> QNVGKWGPMVKFPVVPVAVALVPETGNLLVWSSGWPNRWTTAGNGKTYTSLYNVNTGNISDAIVQNTQHDMFCPGTSLDADGRIIVTGGSSAAKTSVLDFKKGESSPWTPLSNMQISRGYQSSCTTSEGKIFVIGGSFSGAGTRNGEVYDPKANTWTKLAGCPVKPLVMQRGMFPDSHAWLWSWKNGSVLQAGPSKKMNWYDTKGTGSNTPAGLRGTDEDSMCGVSVMYDAVAGKIFTYGGGKGYT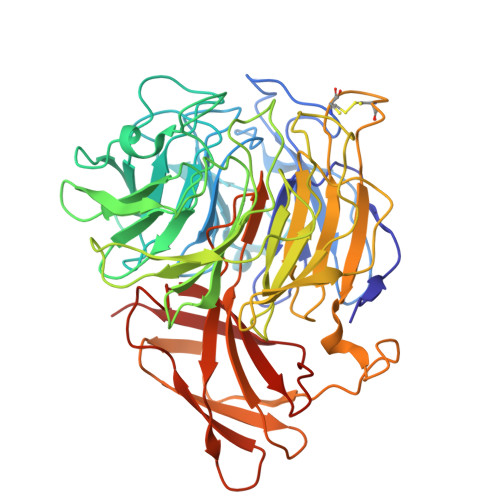GYDSTSNAHILTLGEPGQAVQVQKLANGKYNRGFANAVVMPDGKIWVVGGMQKMWLFSDTTPQLTPELFDPATGSFTPTTPHTVPRNYHSTALLMADATIWSGGGGLCGANCKENHFDGQFWSPPYLFEADGVTPAKRPVIQSLSDTAVRAGAPITITMQDAGAYTFSMIRVSATTHTVNTDQRRIPLDGQDGGDGKSFTVNVPNDYGVAIPGYYMLFAMNEAGVPCVAQFFKVTLHHHHHH>GSAAASSVDTSQEFQNNLKNAIGNLPFQYVNGIYELNNNQTNLNADVNVKAYVQNTIDNQQRPSTANAMLDRTIRQYQNRRDTTLPDANWKPLGWHQVATNDHYGHAVDKGALIAY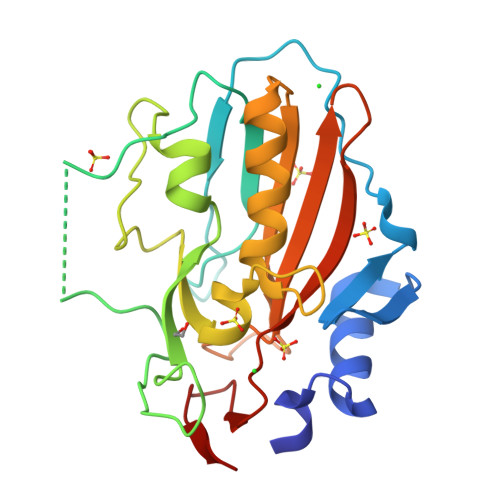ALAGNFKGWDASVSNPQNVVTQTAHSNQSNQKINRGQNYYESLVRKAVDQNKRVRYRVTPLYRNDTDLVPFAMHLEAKSQDGTLEFNVAIPNTQASYTMDYATGEITLN[2x]> AFAHFVLIHTICHGAWIWHKLKPLLEALGHKVTALDL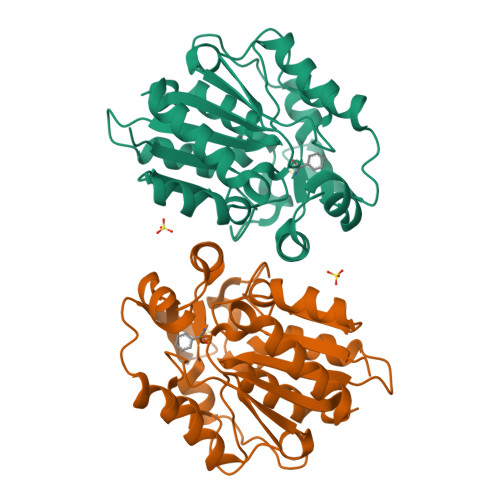AASGVDPRQIEEIGSFDEYSEPLLTFLEALPPGEKVILVGESCGGLNIAIAADKYCEKIAAAVFHNSVLPDTEHCPSYVVDKLMEVFPDWKDTTYFTYTKDGKEITGLKLGFTLLRENLYTLCGPEEYELAKMLTRKGSLFQNILAKRPFFTKEGYGSIKKIYVWTDQDEIFLPEFQLWQIENYKPDKVYKVEGGDHKLQLTKTKEIAEILQEVADTYN> TTALSLPACPEESPLLVGPMLIEFNMPVDLELVAKQNPNVKMGGRYAPRDCVSPHKVAIIIPFRNRQEHLKYWLYYLHPVLQRQQLDYGIYVINQAGDTIFNRAKLLNVGFQEALKDYDYTCFVFSDVDLIPMNDHNAYRCFSQPRHISVAMDKFGFSLPYVQYFGGVSALSKQQFLTINGFPNNYWGWGGEDDDIFNRLVFRGMSISRPNAVVGRCRMIRHSRDKKNEPNPQRFDRIAHTKETMLSDGLNSLTYQVLDVQRYPLYTQITVDIGTPS

Beta-1,4-galactosyltransferase 1 (B4GalT1; EC 2.4.1.38) is a family 7 glycosyltransferase residing in the trans Golgi. In the presence of manganese, it transfers a galactose moiety (Gal) from UDP-galactose (UDP-Gal) to an N-acetylglucosamine (GlcNAc) residue, with the formation of a β1–4 linkage. B4GalT1 possesses a type II membrane protein topology, with a short N-terminal cytoplasmic tail and an α-helical transmembrane domain responsible for Golgi localization, a stem domain (amino acids 45–125), that is believed to be mostly disordered and whose function is still unknown, and a globular catalytic domain (amino acids 126–398) carrying the sugar transfer activity. Previous structure-function studies of the catalytic domain of B4GalT1 by x-ray crystallography revealed that the enzyme undergoes conformational changes upon substrate binding and during its catalytic cycle.

In the present work we used the wild-type human B4GalT1 and our construct is longer than the previously studied ones (Asp99-Ser398 instead of Ser126-Ser398). It contains a piece of the stem domain (Asp99-Leu125) in addition to the catalytic domain (Ser126-Ser398). We obtained two crystals with distinctly different shapes in the same crystallization conditions. In our open conformation structure of the human wild-type B4GalT1, the lid region, the most prominent ligand binding-controlling structural element, is detectable in its entirety. This was not the case in previously published structures of human open B4GalT1, containing mutations R337T, C338T and M340H. However, comparison of the lid positions can be made with the bovine open B4GalT1 structure, for which all residues could be traced in the electron density map. Even though the proteins have crystallized in different space groups and unit cells and the packing of molecules is different, the lid is observed in a similar orientation, except for residues 346–352, which are slightly displaced (RMSD ≈ 2.5 Å, data not shown). One noteworthy difference which is functionally important for ligand binding, is that in our open structure, Trp310 has a new and unexpected orientation with an RMSD of ≈ 2.0 Å compared with human closed structure. The Trp loop in the open structure lies in the vicinity of His361 and Tyr307 and makes short distance (<3.8Å) hydrophobic contacts with those residues as well as long range (≈7Å) hydrophobic contacts with Phe356.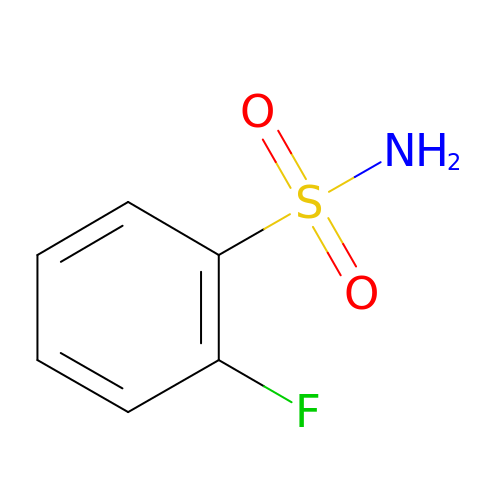2-fluorobenzenesulfonamide | C6 H6 F N O2 S | WFLBWYLZCQOPCA-UHFFFAOYSA-N> MSIFTIFISALLVNNFVLSRFLGICPFLGVSKKVETA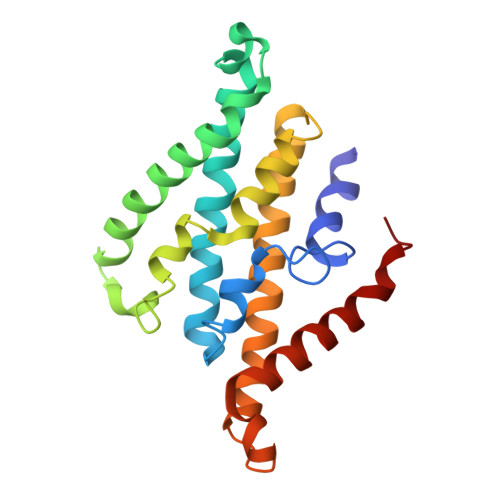TGMGAAVTFVMALAAIMTFLVERFILIPLNIQYLSTLAFILVIASLVQFVEMVIKKVSPDLYKALGIYLPLITTNCAVLGMAVINSNEKYNLIQSIINSVGAALGFTLALVLLAGIREKMETNEYIPEALKGLPITLVTAGLMAIAFLGFQGLI> SEISRQEFQRRRQALVEQMQPGSAALIFAAPEVTRSADSEYPYRQNSDFWYFTGFNEPEAVLVLIKSDDTHNHSVLFNRVRDLTAEIWFGRRLGQDAAPEKLGVDRALAFSEINQQLYQLLNGLDVVYHAQGEYAYADVIVNSALEKLRKGSRQNLTAPATMIDWRPVVHEMRLFKSPEEIAVLRRAGEITAMAHTRAMEKCRPGMFEYHLEGEIHHEF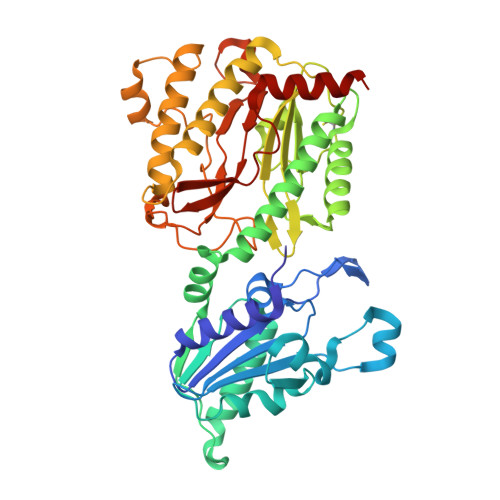NRHGARYPSYNTIVGSGENGCILAYTENECEMRDGDLVLIDAGCEYKGYAGDITRTFPVNGKFTQAQREIYDIVLESLETSLRLYRPGTSILEVTGEVVRIMVSGLVKLGILKGDVDELIAQNAHRPFFMHGLSHWLGLDVHDVGVYGQDRSRILEPGMVLTVEPGLYIAPDAEVPEQYRGIGIRIEDDIVITETGNENLTASVVKKPEEIEALMVAARKQ>[6x]MGSSHHHHHHH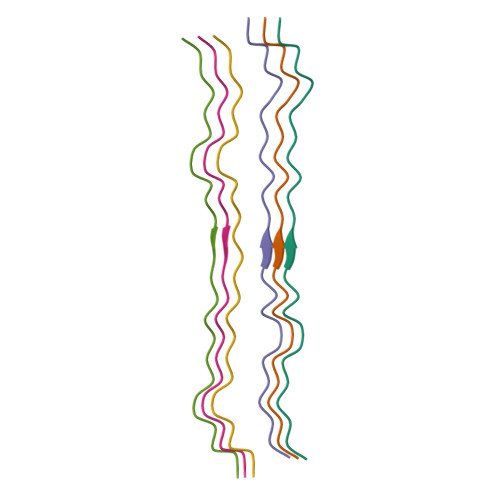HHHHHSENLYFQGGQYMPNGWQVPAYGMYGQAWNQQGFNQTQSSAPWMGPNYGVQPPQGQNGSMLPNQPSGYRVAGYETQ> MKYSQCLKGEVVMIPALAKKILHVTVGTLLVSSAASMMVYLNSMCHMAANSKTQQIQGDDNKDDKFPLASISKVVTTLWAVDRLGPDYRF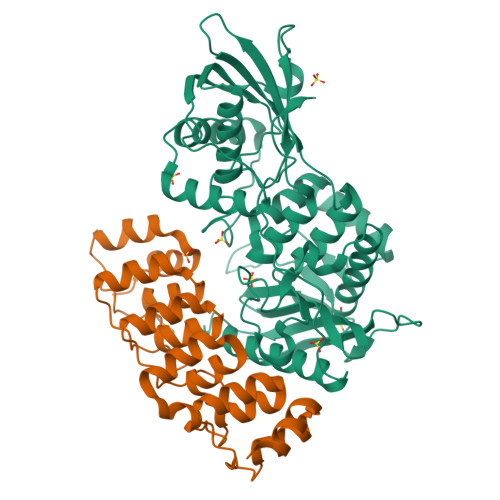KTKLHVTPTANGSYDIHIEGSRDPLFGRNMSYFLISELNRMKITKIEKLTFDENFLLAWLAEEKPMIGGTTPKYDTVEQQASIVRATLTSSFATAISPGYYTILKTKAARIGVQMSNRPKIDVRTISFVKKAEFQKNEKSTTMVLMSAPLKTILKRMNNQSNNYIADNLYWNLGGTEAFNAYIAGKMQADTSDIEFHNGSGNNEGSVAKPVYNEATCEMMIKVLYSLDKSLSAKGYDLSDVMAVAAKDKASTVGSYGGVMAGSTTAKTGSVNKAKTLMGSVSTKNGEIYFAVLMHTDYDKSRSDWGVASQQIKNKVSQLINQNGGPKAIKYTEQLPLPFDKYSYLTKANTITTEKK;> MKKSYLLAALIFFLAGLLHGTAFAMSGKSSKALNEAAEQGDLAKVKNLVQKNKIDLNAQDETGMTPLMNAAMGGNLDIVKFLLSKKVNLELKNNGGETALAFAVTNDAYDVAEELIKAGANVDIIVAGDEGDTLFMRAAQNNKKTAESILAKNKSLINKANTLGETALFAVARYGTPADIDFLIKKGADLKLKNKKGQTALDVAKEASNQDTAKALSKKKLEHHHHHHHH> MDAYSTRPLTLSHGSLEHVLLVPTASFFIASQLQEQFNKILPEPTEGFAADDEPTTPAELVGKFLGYVSSLVEPSKVGQFDQVLNLCLTEFENCYLEGNDIHALAAKLLQENDTTLVKTKELIKNYITARIMAKRPFDKKSNSALFRAVGEGNAQLVAIFGGQGNTDDYFEELRDLYQTYHVLVGDLIKFSAETLSELIRTTLDAEKVFTQGLNILEWLENPSNTPDKDYLLSIPISCPLIGVIQLAHYVVTAKLLGFTPGELRSYLKGATGHSQGLVTAVAIAETDSWESFFVSVRKAITVLFFIGVRCYEAYPNTSLPPSILEDSLENNEGVPSPMLSISNLTQEQVQDYVNKTNSHLPAGKQVEISLVNGAKNLVVSGPPQSLYGLNLTLRKAKAPSGLDQSRIPFSERKLKFSNRFLPVASPFHSHLLVPASDLINKDLVKNNVSFNAKDIQIPVYDTFDGSDLRVLSGSISERIVDCIIRLPVKWETTTQFKATHILDFGPGGASGLGVLTHRNKDGTGVRVIVAGTLDINPDDDYGFKQEIFDVTSNGLKKNPNWLEEYHPKLI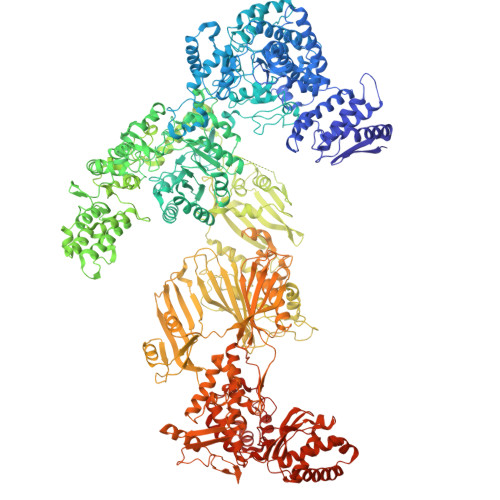KNKSGKIFVETKFSKLIGRPPLLVPGMTPCTVSPDFVAATTNAGYTIELAGGGYFSAAGMTAAIDSVVSQIEKGSTFGINLIYVNPFMLQWGIPLIKELRSKGYPIQFLTIGAGVPSLEVASEYIETLGLKYLGLKPGSIDAISQVINIAKAHPNFPIALQWTGGRGGGHHSFEDAHTPMLQMYSKIRRHPNIMLIFGSGFGSADDTYPYLTGEWSTKFDYPPMPFDGFLFGSRVMIAKEVKTSPDAKKCIAACTGVPDDKWEQTYKKPTGGIVTVRSEMGEPIHKIATRGVMLWKEFDETIFNLPKNKLVPTLEAKRDYIISRLNADFQKPWFATVNGQARDLATMTYEEVAKRLVELMFIRSTNSWFDVTWRTFTGDFLRRVEERFTKSKTLSLIQSYSLLDKPDEAIEKVFNAYPAAREQFLNAQDIDHFLSMCQNPMQKPVPFVPVLDRRFEIFFKKDSLWQSEHLEAVVDQDVQRTCILHGPVAAQFTKVIDEPIKSIMDGIHDGHIKKLLHQYYGDDESKIPAVEYFGGESPVDVQSQVDSSSVSEDSAVFKATSSTDEESWFKALAGSEINWRHASFLCSFITQDKMFVSNPIRKVFKPSQGMVVEISNGNTSSKTVVTLSEPVQGELKPTVILKLLKENIIQMEMIENRTMDGKPVSLPLLYNFNPDNGFAPISEVMEDRNQRIKEMYWKLWIDEPFNLDFDPRDVIKGKDFEITAKEVYDFTHAVGNNCEDFVSRPDRTMLAPMDFAIVVGWRAIIKAIFPNTVDGDLLKLVHLSNGYKMIPGAKPLQVGDVVSTTAVIESVVNQPTGKIVDVVGTLSRNGKPVMEVTSSFFYRGNYTDFENTFQKTVEPVYQMHIKTSKDIAVLRSKEWFQLDDEDFDLLNKTLTFETETEVTFKNANIFSSVKCFGPIKVELPTKETVEIGIVDYEAGASHGNPVVDFLKRNGSTLEQKVNLENPIPIAVLDSYTPSTNEPYARVSGDLNPIHVSRHFASYANLPGTITHGMFSSASVRALIENWAADSVSSRVRGYTCQFVDMVLPNTALKTSIQHVGMINGRKLIKFETRNEDDVVVLTGEAEIEQPVTTFVFTGQGSQEQGMGMDLYKTSKAAQDVWNRADNHFKDTYGFSILDIVINNPVNLTIHFGGEKGKRIRENYSAMIFETIVDGKLKTEKIFKEINEHSTSYTFRSEKGLLSATQFTQPALTLMEKAAFEDLKSKGLIPADATFAGHSLGEYAALASLADVMSIESLVEVVFYRGMTMQVAVPRDELGRSNYGMIAINPGRVAASFSQEALQYVVERVGKRTGWLVEIVNYNVENQQYVAAGDLRALDTVTNVLNFIKLQKIDIIELQKSLSLEEVEGHLFEIIDEASKKSAVKPRPLKLERGFACIPLVGISVPFHSTYLMNGVKPFKSFLKKNIIKENVKVARLAGKYIPNLTAKPFQVTKEYFQDVYDLTGSEPIKEIIDNWEKYEQSDYKDHDGDYKDHDIDYKDDDDK>MRGGALLCGQVQDEIEQLSRESSHFSLSTGILPSLGARSNRRVKLRRFVVSPYDHKYRIWEAFLVVLVVYTAWVSPFEFGFLRKPRPPLSITDNIVNAFFAIDIIMTFFVGYLDKSTYLIVDDRKQIAFKYLRSWFLLDLVSTIPSEAAMRISSQSYGLFNMLRLWRLRRVGALFARLEKDRNFNYFWVRCAKLVCVTLFAVHCAACFYYLIAARNSNPAKTWIGANVANFLEESLWMRYVTSMYWSITTLTTVGYGDLHPVNTKEMIFDIFYMLFNLGLTAYLIGNMTNLVVHGTSRTRNFRDTIQAASNFAHRNHLPPRLQDQMLAHLCLKYRTDSEGLQQQETLDALPKAIRSSISHFLFYSLMDKVYLFRGVSNDLLFQLVSEMKAEYFPPKEDVILQNEAPTDFYILVNGTADLVDVDTGTESIVREVKAGDIIGEIGVLCYRPQLFTVRTKRLCQLLRMNRTTFLNIIQANVGDGTIIMNNLLQHLKEMNDPVMTNVLLEIENMLARGKMDLPLNLCFAAIREDDLLLHQLLKRGLDPNESDNNGRTPLHIAASKGTLNCVLLLLEYHADPNCRDAEGSVPLWEAMVEGHEKVVKVLLEHGSTIDAGDVGHFACTAAEQGNLKLLKEIVLHGGDVTRPRATGTSALHTAVCEENIEMVKYLLEQGADVNKQDMHGWTPRDLAEQQGHEDIKALFREKLHERRVHIETSSSVPILKTGIRFLGRFTSEPNIRPASREVSFRIRETRARRKTNNFDNSLFGILANQSVPKNGLATVDEGRTGNPVRVTISCAEKDDIAGKLVLLPGSFKELLELGSNKFGIVATKVMNKDNNAEIDDVDVIRDGDHLIFATDSLEGSDEVDAGSAAASGGSGSDYKDDDDK[2x];>MSTTTTEARSPLPLLLRRGRSSTALSASTAEARSPLSILQFRRRSSKDVRNITSVSSSLLPAFGTFIEDDNPSSKPFIVLHFDRRYRLWELFLVILVGYSAWASLFELAFEKAAEGALLTIDLVVDFFFAVDIILTFFVSYLDNTTYLNVTDHKLIAKRYLKSVAFVMDVASTLPIQ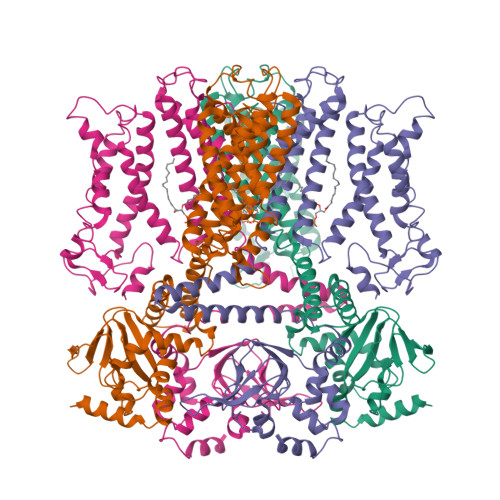FIYKTITGDVGRGQAFGFLNLLRLWRLRRVAELFKRLEKDAHFNYFVIRVIKLLCVTIFWIHLAGCILYWIAYHYPRPTDTWIGSQVEDFKERSVWLGYTYSMYWSIVTLTTVGYGDLHAVNSREKTFNMFYMLFNIGLTSYIIGIMTNLVVHGALRTFAMRSAINDILRYTSKNRLPDTMREQMLAHMQLKFKTAELRQEEVLQDLPKAIRSSINQHLFRSIIEEAYLFKGFPEGLLVQLVSQIQAEYFPPKMEIILQNEIPTDFYVIVSGGVDIIASKGVSEQVLAKLGPGSMAGEIGVVFNIPQPFTVRTRRLSQVIRIGHHKFKEMVQSDNDVDAKMIIANFMTYLKGLNDELKKEIPFLRDLLDDADAQVQETVQSEETPQSNDEEIVTVSRHENGQIEERRREGVPKRVIIHGQAPPNQDNKNNGDSNGRLIILPDSIQLLFDLAEKKLGKRGSTIAMADGAHVEQIDALRENDHLYIFLEGSDEVDAGSAAASGGSGSWSHPQFEK[2x]GUANOSINE-3',5'-DIPHOSPHATE | C10 H15 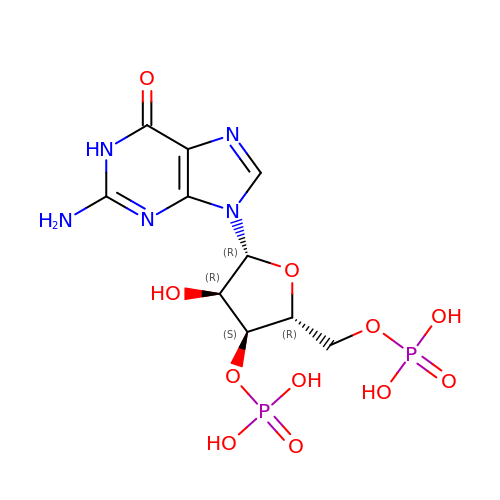N5 O11 P2 | XYVNHPYNSPGYLI-UUOKFMHZSA-N> MAMHPRKDWYELTRATNWTPSYVTEEQLFPERMSGHMGIPLEKWESYDEPYKTSYPEYVSIQREKDAGAYSVKAALERAKIYENSDPGWISTLKSHYGAIAVGEYAAVTGEGRMARFSKAPGNRNMATFGMMDELRHGQLQLFFPHEYCKKDRQFDWAW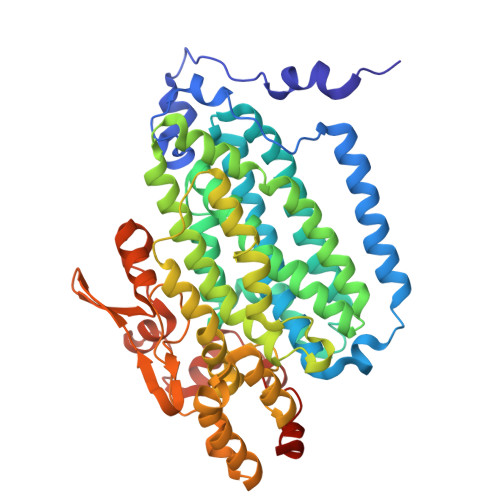RAYHSNEWAAIAAKHFFDDIITGRDAISVAIMLTFSFETGFTNMQFLGLAADAAEAGDYTFANLISSIQTDESRHAQQGGPALQLLIENGKREEAQKKVDMAIWRAWRLFAVLTGPVMDYYTPLEDRSQSFKEFMYEWIIGQFERSLIDLGLDKPWYWDLFLKDIDELHHSYHMGVWYWRTTAWWNPAAGVTPEERDWLEEKYPGWNKRWGRCWDVITENVLNDRMDLVSPETLPSVCNMSQIPLVGVPGDDWNIEVFSLEHNGRLYHFGSEVDRWVFQQDPVQYQNHMNIVDRFLAGQIQPMTLEGALKYMGFQSIEEMGKDAHDFAWADKCKPAMKKSA>[2x]RKPKTGILMLNMGGPETLGDVHDFLLRLFLDRDLMTLPIQNKLAPAIAKRRTPKIQEQYRRIGGGSPIKIWTSKQGEGMVKLLDELSPNTAPHKYYIGFRYVHPLTEEAIEEMERDGLERAIAFTQYPQYSCSTTGSSLNAIYRYYNQVGRKPTMKWSTIDRWPTHHLLIQCFADHILKELDHFPLEKRSEVVILFSAHSLPMSVVNRGDPYPQEVSATVQKVMERLEYCNP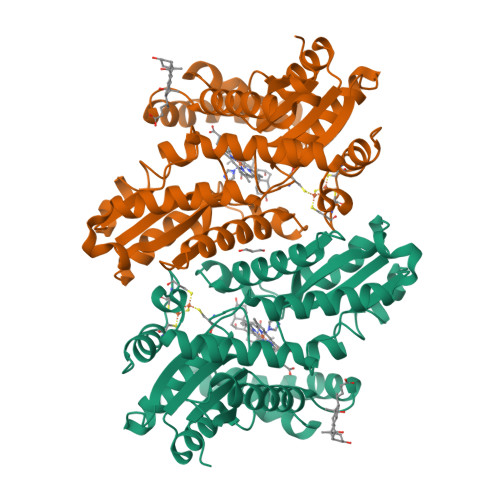YRLVWQSKVGPMPWLGPQTDESIKGLCERGRKNILLVPIAFTSDHIETLYELDIEYSQVLAKECGVENIRRAESLNGNPLFSKALADLVHSHIQSNELCSKQLTLSCPLCVNPVCRETKSFFTSQQL>[2x]HHHHHHFNLPPGNYKKPKLLYCSNGGHFLRILPDG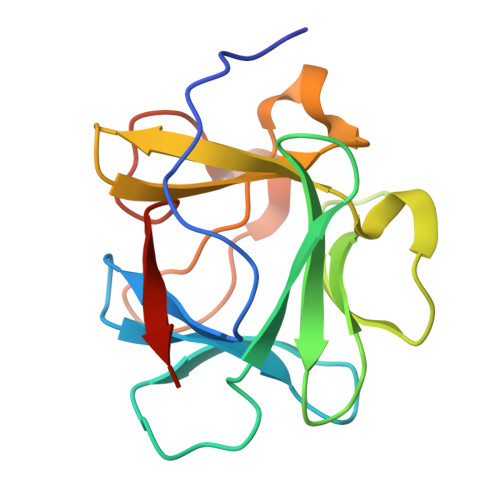TVDGTRDRSDQHIQLQLSAESVGEVYIKSTETGQYLAMDTDGLLYGSQTPNEECLFLERLEENHYNTYISKKHAEKNWFLGLKKNGSCKRGPRTHYGQKAILFLPLPVSSD>ADNLAEFHVQNQECDSCHTPDGELSNDSLTYENTQCVSCHGTLAEVAETTKHEHYNAHASHFPGEVACTSCHSAHEKSMVYCDSCHSFDFNMPYAKKWLRDEPTIAELAKDKSERQAALASAPHDTVDVVVVGSGGAGFSAAISATDSGAKVILIEKEPVIGGNAKLAAGGMNAAWTDQQKAKKITDSPELMFEDTMKGGQNINDPALVKVLSSHSKDSVDWMTAMGADLTDVGMMGGASVNRAHRPTGGAGVGAHVVQVLYDNAVKRNIDLRMNTRGIEVLKDDKGTVKGILVKGMYKGYYWVKADAVILATGGFAKNNERVAKLDPSLKGFISTNQPGAVGDGLDVAENAGGALKDMQYIQAHPTLSVKGGVMVTEAVRGNGAILV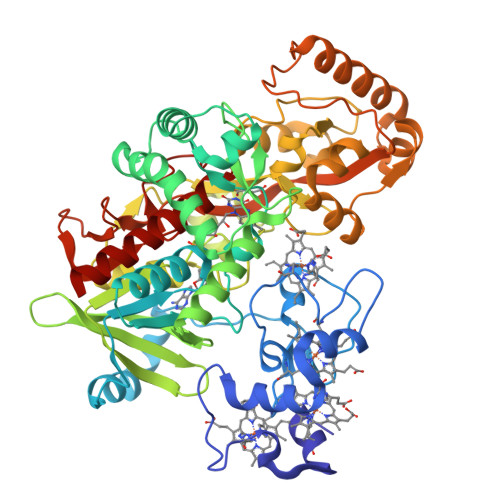NREGKRFVNEITTADKASAAILAQTGKSAYLIFDDSVRKSLSKIDKYIGLGVAPTADSLVKLGKMEGIDGKALTETVARYNSLVSSGKDTDFERPNLPRALNEGNYYAIEVTPGVHHTMGGVMIDTKAEVMNAKKQVIPGLYGAGEVTGGVHGANRLGGNAISDIITFGRLAGEEAAKYSKKN[2x]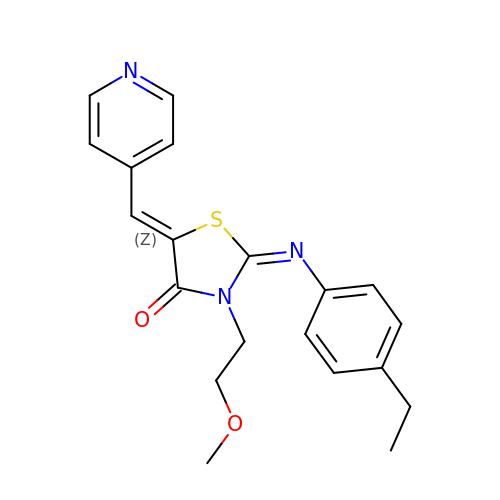(2Z,5Z)-2-[(4-ethylphenyl)imino]-3-(2-methoxyethyl)-5-(pyridin-4-ylmethylidene)-1,3-thiazolidin-4-one | C20 H21 N3 O2 S | NNYRUSJDMFVRJF-JHRGVAJVSA-N>MALTQVETEIVPVSVDGETLTVEAVRRVAEERATVDVPAESIAKAQKSREIFEGIAEQNIPIYGVTTGYGAMIYMQVDKSKEVELQTNLVRSHSAGVGPLFAEDEARAIVAARLNTLAKGHSAVRPIILERLAQYLNEGITPAIPEIGSLGASGDLAPLSHVASTLIGEGYVLRDGRPVETAQVLAERGIEPLELRFKEGLALINGTSGMTGLGSLVVGRALEQAQQAEIVTALLIEAVRGSTSPFLAEGHDIARPHEGQIDTAANMRALMRGSGLTVEHADLRRELQKDKEAGKDVQRSEIYLQKAYSLRAIPQVVGAVRDTLYHARHKLRIELNSANDNPLFFEGKEIFHGANFHGQPIAFAMDFVTIALTQLGVLAERQINRVLNRHLSYGLPEFLVSGDPGLHSGFAGAQYPATALVAENRTIGPASTQSVPSNGDNQDVVSMGLISARNARRVLSNNNKILAVEYLAAAQAVDISGRFDG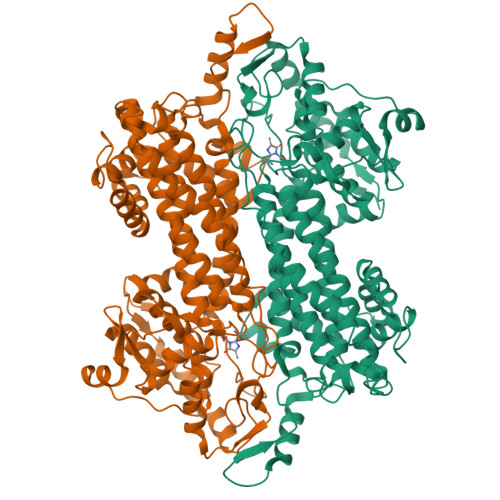LSPAAKATYEAVRRLVPTLGVDRYMADDIELVADALSRGEFLRAIARETDIQLR[2x]> DICPASEDESGQWKNFRLPDFVNPVHYDLHVKPLLEEDTYTGTVSISINLSAPTRYLWLHLRETRITRLPELKRPSGDQVQVRRCFEYKKQEYVVVEAEEELTPSSGDGLYLLTMEFAGWLNGSLVGFYRTTYTENGRVKSIAATDHEPTDARKSFPCFDEPNKKATYTISITHPKEYGALSNMPVAKEESVDDKWTRTTFEKSVPMSTYLVCFAVHQFDSVKRISNSGKPLTIYVQPEQKHTAEYAANITKSVFDYFEEYFAMNYSLPKLDKIAIPDFGTGAMENWGLITYRETNLL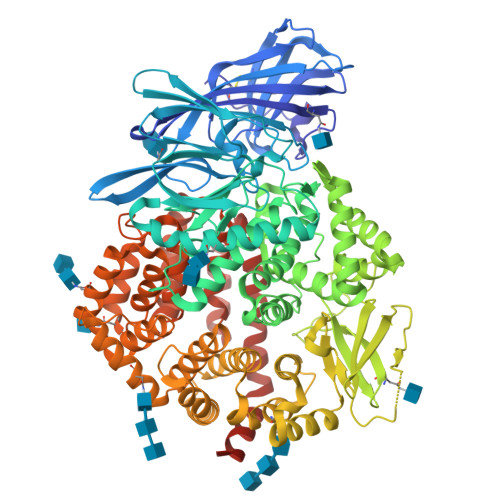YDPKESASSNQQRVATVVAHELVHQWFGNIVTMDWWEDLWLNEGFASFFEFLGVNHAETDWQMRDQMLLEDVLPVQEDDSLMSSHPIIVTVTTPDEITSVFDGISYSKGSSILRMLEDWIKPENFQKGCQMYLEKYQFKNAKTSDFWAALEEASRLPVKEVMDTWTRQMGYPVLNVNGVKNITQKRFLLDPRANPSQPPSDLGYTWNIPVKWTEDNITSSVLFNRSEKEGITLNSSNPSGNAFLKINPDHIGFYRVNYEVATWDSIATALSLNHKTFSSADRASLIDDAFALARAQLLDYKVALNLTKYLKREENFLPWQRVISAVTYIISMFEDDKELYPMIEEYFQGQVKPIADSLGWNDAGDHVTKLLRSSVLGFACKMGDREALNNASSLFEQWLNGTVSLPVNLRLLVYRYGMQNSGNEISWNYTLEQYQKTSLAQEKEKLLYGLASVKNVTLLSRYLDLLKDTNLIKTQDVFTVIRYISYNSYGKNMAWNWIQLNWDYLVNRYTLNNRNLGRIVTIAEPFNTELQLWQMESFFAKYPQAGAGEKPREQVLETVKNNIEWLKQHRNTIREWFFNLLESGHHHHHH> DWVIPPISSPENEKGPFPKNLVQIKSNKDKEGKVFYSITGQGADTPPVGVFIIERETGWLKVTEPLDRERIATYTLFSHAVSSNGNAVEDPMEILITVTDQNDNKPEFTQEVFK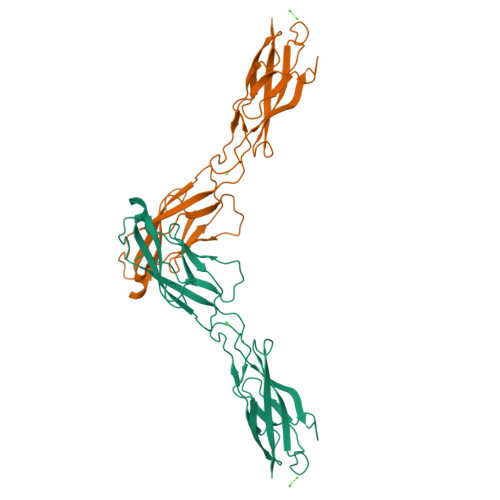GSVMEGALPGTSVMEVTATDADDDVNTYNAAIAYTILSQDPELPDKNMFTINRNTGVISVVTTGLDRESFPTYTLVVQAADLQGEGLSTTATAVITVTD> ETGSAQQLNEDLRLHLLLNTSVTCNDGSPAGYYLKESRGSRRWLLFLEGGWYCFNRENCDSRYDTMRRLMSSRDWPRTRTGTGILSSQPEENPYWWNANMVFIPYCSSDVWSGASSKSEKNEYAFMGALIIQEVVRELLGRGLSGAKVLLL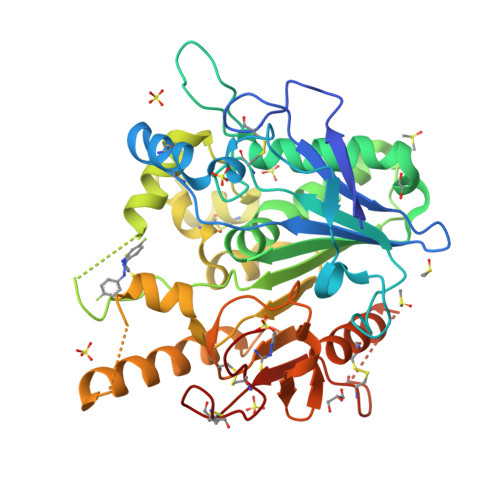AGSSAGGTGVLLNVDRVAEQLEKLGYPAIQVRGLADSGWFLDNKQYRHTDCVDTITCAPTEAIRRGIRYWNGVVPERCRRQFQEGEEWNCFFGYKVYPTLRSPVFVVQWLFDEAQLTVDNVHLTGQPVQEGLRLYIQNLGRELRHTLKDVPASFAPACLSHEIIIRSHWTDVQVKGTSLPRALHCWDRSLHDSHKASKTPLKGCPVHLVDSCPWPHCNPSCPTGTHHHHHH methyl 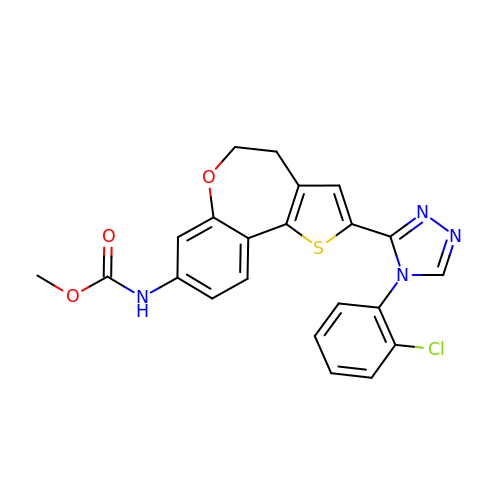{2-[4-(2-chlorophenyl)-4H-1,2,4-triazol-3-yl]-4,5-dihydrothieno[3,2-d][1]benzoxepin-8-yl}carbamate | C22 H17 Cl N4 O3 S | IMSBGZSMSGCJBM-UHFFFAOYSA-N> MRSKYIVIEGLEGAGKTTARNVVVE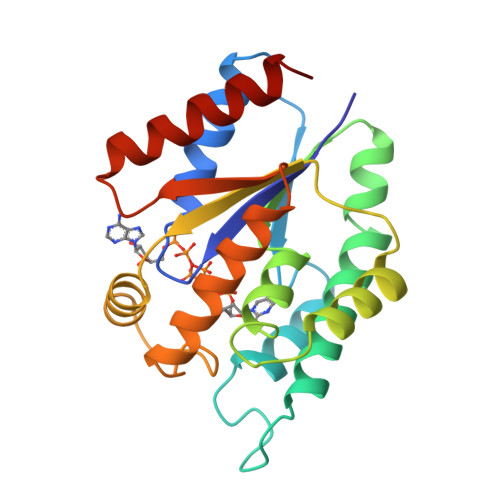TLEQLGIRDMVFTREPGGTQLAEKLRSLLLDIKSVGDEVITDKAEVLMFYAARVQLVETVIKPALANGTWVIGDRHDLSTQAYQGGGRGIDQHMLATLRDAVLGDFRPDLTLYLDVTPEVGLKRARARGELDRIEQESFDFFNRTRARYLELAAQDKSIHTIDATQPLEAVMDAIRTTVTHWVKELDA2,6-difluoro-N-[1-(5-{[2-(4-fluorophenoxy)ethyl]sulfanyl}-4-methyl-4H-1,2,4-triazol-3-yl)ethyl]benzamide 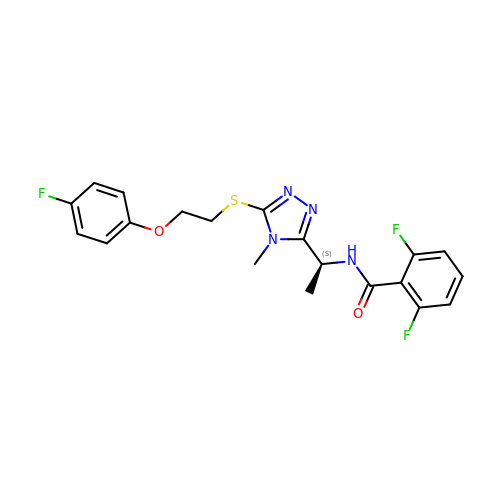| C20 H19 F3 N4 O2 S | OUIZIUPLGXONEI-LBPRGKRZSA-N>[2x]MDSIQAEEWYFGKIT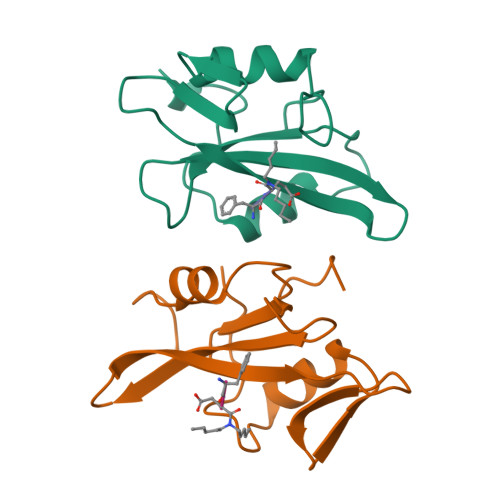RRESERLLLNAENPRGTFLVRESETTKGAYCLSVSDFDNAKGLNVKHYKIRKLDSGGFYITSRTQFNSLQQLVAYYSKHADGLCHRLTTVCP>MRKAVSQRNKLILWTRGGGRCYLCNCALLGDLISGKDKLNKGYIAHIVAAEIDGPRGDPIRSPLLCDDVENLILLCDAHHRLIDVEAVAEYSEPRLQQIKRAHEARVEAVTEITADRGTHMLFYSARIGEHDCPIQAQDARSAVLPAYYPKDRHPIALDVARSEYADNEAQYWQFQIENLNRQFERKVRPLLADGHIDHLSVFGLAPQPLLIHLGRLLSDLRKVRVHQLHREPKGWDWRNERPPVVYKTDRTGHGRTIALKIGISATIVDERITRCLGEDTTIWSLSAEGAHNDILHSEGDLQTFRSTCRRLFDAIKAAHPDATDLHIFPAMPVSTAIELGRIWMPKADLPLHIYDENRTAGGFFHRHSLGGVSIPKTEEPIYG[2x]

Here, we present the biochemical and structural characterization of two CBASS systems, composed of CdnG and Cap5, from Asticcacaulis sp. and Lactococcus lactis. We show that CdnG from Asticcacaulis sp. synthesizes 3′,2′-cGAMP in vitro, and 3′,2′-cGAMP is the biological signaling molecule that activates Cap5 for DNA degradation. Each monomer of Cap5 is composed of the N-terminal HNH domain, the C-terminal SAVED domain, and a short flexible linker connecting these two domains. The structures revealed that both Cap5 form homodimers, resulting from the side-by-side packing of two HNH domains.

On the other hand, two SAVED domains in the structure of AsCap5 are close and make contact with one another. But the two contacting surfaces are not completely closed and a gap between them can be seen. Therefore, the structure of AsCap5 can be best described as in ajar configuration. Importantly, unlike the two-fold symmetry applicable for the entire LlCap5 structure, the Front of the first SAVED domain of AsCap5 faces the Back of the second SAVED domain. Therefore, the two-fold symmetry is only applicable to the HNH homodimer. The HNH domain of AsCap5 (AsCap5-HNH) is significantly more structured near the active site than the one of LlCap5. Specifically, a well-coordinated Mg2+ ion is only observed with AsCap5-HNH, and nine residues of LlCap5-HNH near the active site are disordered. We created a model of AsCap5-HNH in complex with DNA•RNA hybrid, which revealed that part of a loop in AsCap5-HNH has a steric clash with the DNA strand of the modeled DNA•RNA hybrid (colored black). Based on this analysis, we conclude that the configuration of AsCap5 shown in Fig. 3b is also likely to be inactive. 3′,2′-cGAMP might act as a glue, bringing two SAVED domains closer to seal the gap shown in the structure of AsCap5 (right).Here, we reported the enzymatic characterizations and crystal structures of marine bacterial esterases CrmE10 and AlinE4. The results showed that both CrmE10 and AlinE4 belong to the SGNH-hydrolase superfamily and the bacterial lipolytic enzyme GDSL family. The SGNH-hydrolase family, a superfamily that includes the bacterial lipolytic enzyme GDSL family, consists of enzymes possessing four strictly conserved residues, Ser, Gly, Asn, and His, in four conserved blocks, I, II, III, and V, respectively. Among these four residues, Ser and His serve as catalytic residues, and Ser, Gly, and Asn serve as oxyanion hole residues.

According to sequence alignment, the catalytic triad of CrmE10 consisted of Ser29, Asp178, and His181, and it was composed of Ser13, Asp162, and His165 in AlnE4. In mutants AlinE4-S13A, AlinE4-D162A, and AlinE4-H165A, catalytic activities toward p-NP esters were almost abolished. In this reaction, Ser is a nucleophile residue, and His is the proton donor/acceptor. In SGNH-hydrolase family enzymes, the residue Ser on the catalytic triad was considered an essential element for aromatic acyl substrate binding, and His was considered as the proton donor/acceptor.

> SMGESRVILAFGDALFAGYGLDKGESYPAKLETALRSHGINARIINAGVSGDTTAAGLQRIKFVLDSQPDKPELAIVELGGNDLLRGLSPAEARQNLSGILEELQRRKIPILLMGMRAPPNLGAKYQREFDGIYPYLAEKYDAKLVPFFLEAVADRPDLIQKDHVHPTARGVEELVSATSNAVAKALPAKK Dihydroflavonol 4-reductase (DFR) and flavanone 4-reductase (FNR) reduce dihydroflavonols and flavanones, respectively, using NAD(P)H to produce flavan-(3)-4-(di)ols in flavonoid biosynthesis. Anthocyanidin reductase (ANR) reduces anthocyanidins to flavan-3-ols. In addition to their sequences, the 3D structures of recombinant DFR, FNR and ANR from sorghum and switchgrass showed a high level of similarity. The catalytic mechanism, substrate-specificity and key residues of three reductases were deduced from crystal structures, site-directed mutagenesis, molecular docking, kinetics, and thermodynamic ana-lyses.

From the early stages of refinement, a difference (Fo–Fc) electron density map clearly indicated the presence of an NADP+ molecule in the binding pocket of PvDFRa, SbFNR1, and SbFNR2 with its nicotinamide moiety properly positioned for the pro-R hydride transfer towards the catalytic site. The bound nicotinamide ring in PvDFRa, SbFNR1, and SbFNR2 established a syn-conformation, whereas the adenine ring adopted an anti-conformation. However, the crystalized SbFNRs did not display any NADP+, thus had to be added for co-crystallization, which indicated that PvDFRa had a higher affinity for NADP+ than SbFNRs, as confirmed by our ITC results. Having both apo- and NADP(H)-bound forms allowed us to observe the conformational change upon binding NADP(H) in the SbFNRs. Compared to the structure without NADP(H), the loop region, 89Val----Pro100 in SbFNR1 (and 89Val----Lys102 in SbFNR2) went through large conformational changes upon binding of NADP(H). Thermodynamic parameters of SbFNR1 were also assayed with ITC for association with NADP+, and it had a Kd of 13.91 µM that indicated a 10-fold decrease in affinity for NADP+ compared to that of PvDFRa as predicted from the crystal structures. In SbFNR1 and SbFNR2, the corresponding catalytic triad is composed of Ser-133/His-173/Lys-177 and Ser-133/Tyr-171/Lys-175, respectively. His-173 is unique for SbFNR1, as all the other compared enzymes including SbFNR2 have tyrosine in that position. In SbFNR1, the 2′ and 3′ hydroxyl groups of the NADPH ribosyl ring were hydrogen bonded only to the sidechain of Lys-177 that was, in turn, indirectly connected to the sidechain Nδ atom of His-173 through two consecutive water molecules. Thus, compared to PvDFRa, the effect of Lys-177 on lowering pKa could be less significant.

>[2x]MSSSAGNKKTMKTACVTGGSGYIGSALIKLLLEKGYAVKTTVRNPDDMEKNSHLKDLQKLGPLTVFRADMDEEGSFDDAVAGCDYVFLVAAPLHFEAQDPEKEQIEPAIQGTLNTMRSCVKAGTVRRVILTSSVAAVYFRPDLLGDGHGHVLDEDSWSDVDFLRAHKPPTWSHCVSKVLLEKEAGRFAEEHGISLVTILPVIVVGAAPAPKARSSIVDCLSMLSGDEAGLAMLRAIQKTSGEVQLVHVDDLCRAELFLAENATANGRYICSRYHPTLVELATFLAQKYPQYGVKPTDFDDEERPRVTMSLEKLIREGFEYKHNTLEEIYDNVVEYGKALGILPY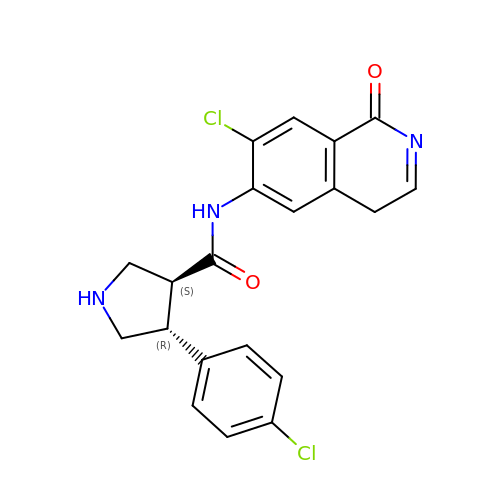(3S,4R)-N-(7-chloro-1-oxo-1,4-dihydroisoquinolin-6-yl)-4-(4-chlorophenyl)pyrrolidine-3-carboxamide | C20 H17 Cl2 N3 O2 | WWMMSIAGRVSGLG-JKSUJKDBSA-N>MSLEPKYQRILIKLSGEALAGEKGVGIDIPTVQAIAKEIAEVHVSGVQI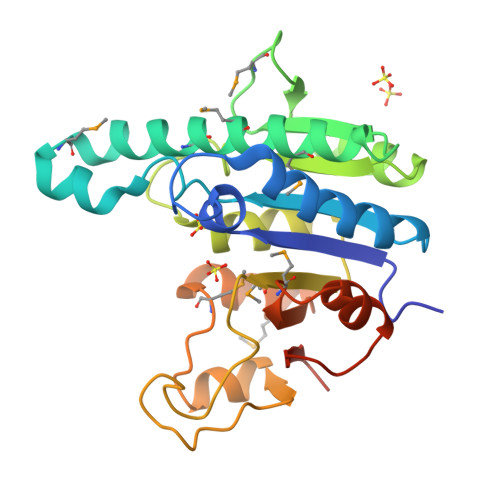ALVIGGGNLWRGEPAADAGMDRVQADYTGMLGTVMNALVMADSLQHYGVDTRVQTAIPMQNVAEPYIRGRALRHLEKNRIVVFGAGIGSPYFSTDTTAALRAAEIEADAILMAKNGVDGVYNADPKKDANAVKFDELTHGEVIKRGLKIMDATASTLSMDNDIDLVVFNMNEAGNIQRVVFGEHIGTTVSNKVCDEGHHHHHH[3x]>[4x]AKEWQENKSWNAHFTEHKSQGVVVLWNENK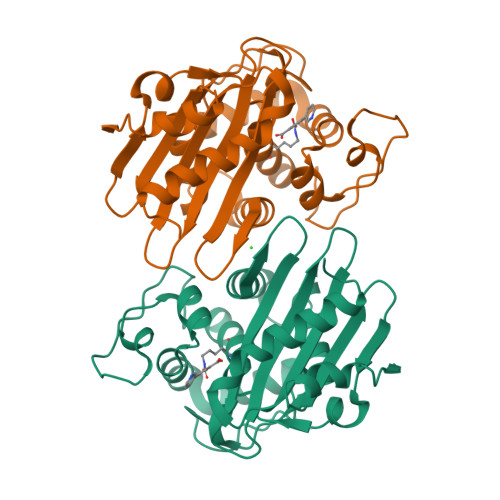QQGFTNNLKRANQAFLPASTFKIPNSLIALDLGVVKDEHQVFKWDGQTRDIATWNRDHNLITAMKYSVVPVYQEFARQIGEARMSKMLHAFDYGNEDISGNVDSFWLDGGIRISATEQISFLRKLYHNKLHVSERSQRIVKQAMLTEANGDYIIRAKTGYSTRIEPKIGWWVGWVELDDNVWFFAMNMDMPTSDGLGLRQAITKEVLKQEKIIP>GQQKNMENKTLNENIPEMIISLEKEALASTDPMAFVELSDTDVIYFDPSLETKIEGLEQLRTYYKGMQLPPADHFDMIRPVVQVAQNIAVLTFNLDSYLSDKVIKWNCTEVYRRNPDNQWKIIQTHWSYVK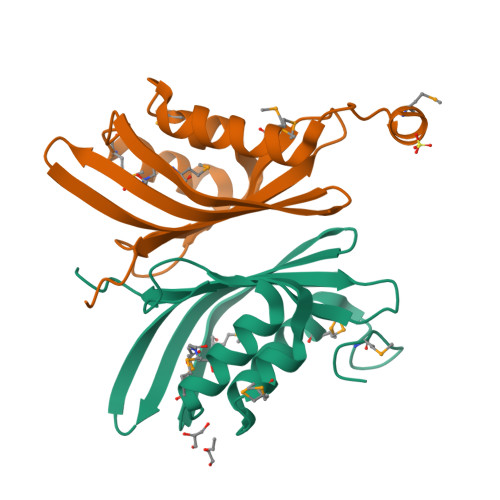PLD[2x]> MRGSHHHHHHGSAQDLTNMPSLAPVLKNAMPAIVNVAVQGYLPNNMASGNADDDDGENSKQPSRIPEKGRKFESIGSGVIIDPKNGIIITNDHVIRNANLITVTLQDGRRLKARLIGGDSETDLAVL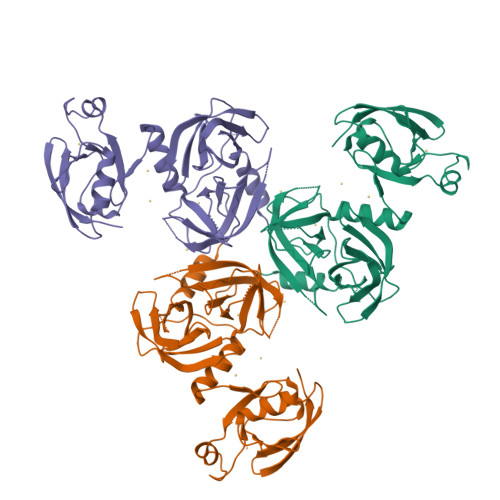KIDAKNLKSLVIGDSDKLEVGDYVVAIGNPFGLNSFGNSQSATFGIVSALKRSDLNIEGVENFIQTDAAINPGNAGGALVNAKGELIGINTAIISPYGGNVGIGFAIPINMAKDVAQQIIKFGSIHRGLMGIFVQHLTPELAQSMGYAEDFQGALVSQVNQNSPAQLAGLKSGDVIVQINDTKITQATQVKTTISLLRAGSTAKIKILRDNKPLTLDVEVTDIK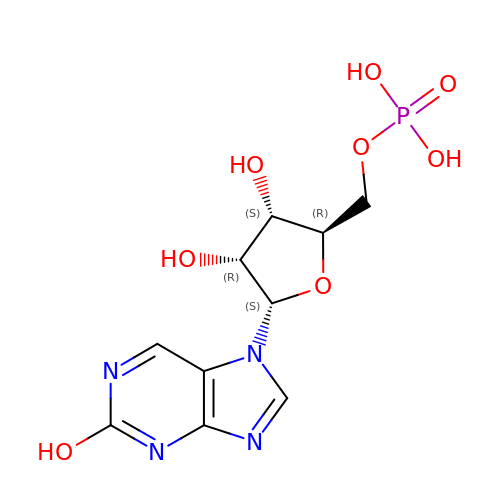N7-(5'-PHOSPHO-ALPHA-RIBOSYL)-2-HYDROXYPURINE | C10 H13 N4 O8 P | BVZASCINAVSQNO-PULFBKJNSA-N>[60x]MILAKVTGHVVATQKCDELRGSNLLLITRLDDKQQPMKDQTWVAVDNVGAGMH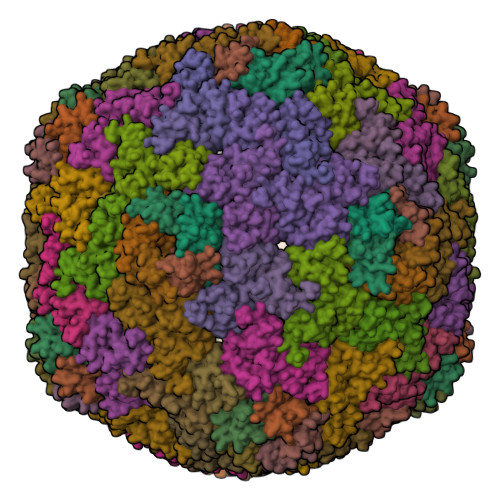DIVLAEEYFALNKDRYKAMSVVAIVEKVFRDTEQE;>[180x]MKEALGLIETKGLVACIEAADAMCKAANVELIGYENVGSGLVTAMVKGDVGAVNAAVDSGVEAAKRIGKVVSSRVIARPHNDIEKIAGSTKHKSLRPHNA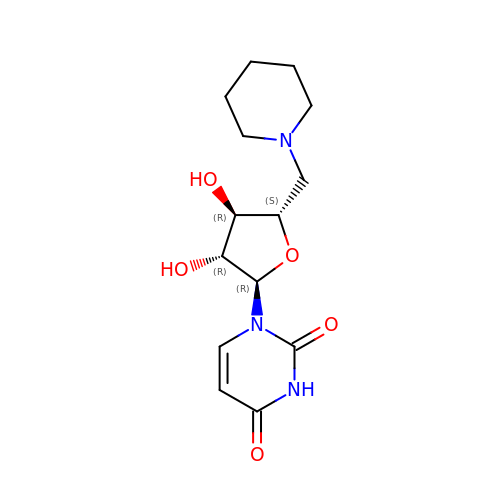1-(5-deoxy-5-piperidin-1-yl-alpha-L-arabinofuranosyl)pyrimidine-2,4(1H,3H)-dione | C14 H21 N3 O5 | PJCAMYRNNJAIMT-FTYKPCCVSA-N Human dipeptidyl peptidase III (hDPP III), also known as enkephalinase B, is a member of the M49 family of zinc dependent metallopeptidases and cleaves dipeptides sequentially from the N-terminus of various bioactive peptide substrates. Crystal structures have so far been determined for DPP III from humans as well as from Saccharomyces cerevisiae. Despite the low sequence identity (36%) shared by the two proteins, both structures are very similar and consist of two lobes separated by a wide cleft. The “upper” lobe is mostly α-helical and contains the zinc binding site as well as the catalytically important residues. In both structures, two histidine residues (His-450 and His-455 in the human enzyme) and a glutamate (Glu-508) coordinate the zinc ion.

We also determined the structure of the unbound enzyme in the closed conformation. As a serendipitous result of the co-crystallization trials we also determined the structure of the unbound enzyme in the closed conformation. As yet, structural studies on human and yeast DPP III in the absence of ligands have always yielded an open extended conformation. Because the crystals in this study were obtained through seeding with microcrystals of an hDPP III ligand complex, it is very likely that this procedure induced crystallization of the protein in the closed conformation.

> MADTQYILPNDIGVSSLDSREAFRLLSPTERLYAYHLSRAAWYGGLAVLLQTSPEAPYIYALLSRLFRAQDPDQLRQHALAEGLTEEEYQAFLVYAAGVYSNMGNYKSFGDTKFVPNLPKEKLERVILGSEAAQQHPEEVRGLWQTCGELMFSLEPRLRHLGLGKEGITTYFSGNCTMEDAKLAQDFLDSQNLSAYNTRLFKEVDGCGKPYYEVRLASVLGSEPSLDSEVTSKLKSYEFRGSPFQVTRGDYAPILQKVVEQLEKAKAYAANSHQGQMLAQYIESFTQGSIEAHKRGSRFWIQDKGPIVESYIGFIESYRDPFGSRGEFEGFVAVVNKAMSAKFERLVASAEQLLKELPWPPTFEKDKFLTPDFTSLDVLTFAGSGIPAGINIPNYDDLRQTEGFKNVSLGNVLAVAYATQREKLTFLEEDDKDLYILWKGPSFDVQVGLHALLGHGSGKLFVQDEKGAFNFDQETVINPETGEQIQSWYRCGETWDSKFSTIASSYEECRAESVGLYLSLHPQVLEIFGFEGADAEDVIYVNWLNMVRAGLLALEFYTPEAFNWRQAHMQARFVILRVLLEAGEGLVTITPTTGSDGRPDARVRLDRSKIRSVGKPALERFLRRLQVLKSTGDVAGGRALYEGYATVTDAPPESFLTLRDTVLLRKESRKLIVQPNTRLEGSDVQLLEYEASAAGLIRSFSERFPEDGPELEEILTQLATADARFW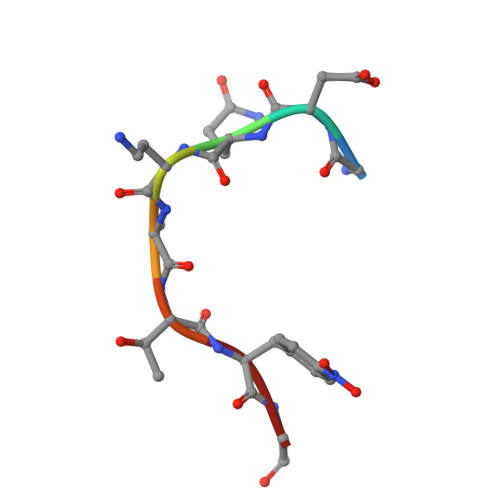> GDQAATFG>CGCGANTTCGCG[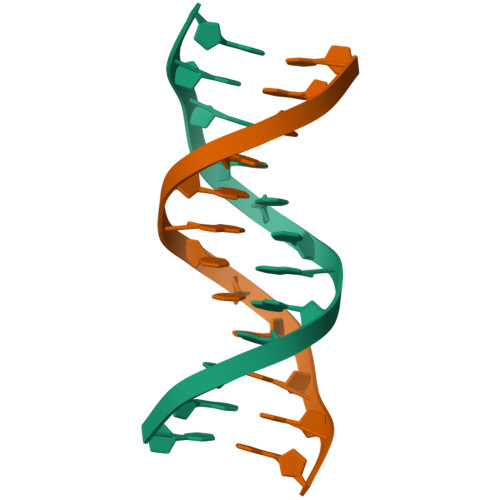2x]> MACLSRIDANLLQYYEKPEPNNTVDLYVSNNSNNNGLKEGDKSISTPVPQPYGSEYSNCLLLSNSEYICYHFSSRSTLLTFYPLSDAYHGKTINIHLPNASMNQRYTLTIQEVEQQLLVNVILKDGSFLTLQLPLSFLFSSANTLNGEWFHLQNPYDFTVRVPHFLFYVSPQFSVVFLEDGGLLGLKKVDGVHYEPLLFNDNSYLKSLTRFFSRSSKSDYDSVISCKLFHERYLIVLTQNCHLKIWDLTSFTLIQDYDMVSQSDSDPSHFRKVEAVGEYLSLYNNTLVTLLPLENGLFQMGTLLVDSSGILTYTFQNNIPTNLSASAIWSIVDLVLTRPLELNVEASYLNLIVLWKSGTASKLQILNVNDESFKNYEWIESVNKSLVDLQSEHDLDIVTKTGDVERGFCNLKSRYGTQIFERAQQILSENKIIMAHNEDEEYLANLETILRDVKTAFNEASSITLYGDEIILVNCFQPYNHSLYKLN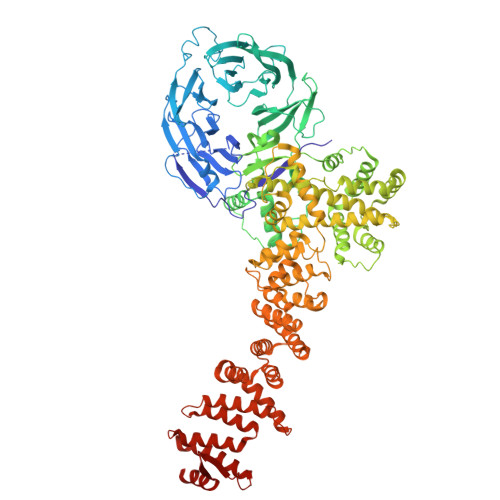TTVENWFYNMHSETDGSELFKYLRTLNGFASTLSNDVLRSISKKFLDIITGELPDSMTTVEKFTDIFKNCLENQFEITNLKILFDELNSFDIPVVLNDLINNQMKPGIFWKKDFISAIKFDGFTSIISLESLHQLLSIHYRITLQVLLTFVLFDLDTEIFGQHISTLLDLHYKQFLLLNLYRQDKCLLAEVLLKDSSEFSFGVKFFNYGQLIAYIDSLNSNVYNASITENSFFMTFFRSYIIENTSHKNIRFFLENVECPFYLRHNEVQEFMFAMTLFSCGNFDQSYEIFQLHDYPEAINDKLPTFLEDLKSENYHGDSIWKDLLCTFTVPYRHSAFYYQLSLLFDRNNSQEFALKCISKSAEYSLKEIQIEELQDFKEKQHIHYLNLLIHFRMFEEVLDVLRLGHECLSDTVRTNFLQLLLQEDIYSRDFFSTLLRLCNAHSDNGELYLRTVDIKIVDSILSQNLRSGDWECFKKLYCFRMLNKSERAAAEVLYQYILMQADLDVIRKRKCYLMVINVLSSFDSAYDQWILNGSKVVTLTDLRDELRGL>[2x]EERKKELAKEVIETAKKLIEKLAKEE

Several natural systems exhibit ‘facilitated dissociation’, in which an effector (E) can bind to a target–host (TH) complex to form an excited ternary complex (THE)20–26 from which the target dissociates quickly. We set out to design protein systems that undergo facilitated dissociation. We use a switchable target binder (host) and a flexible effector that can rapidly bind to and switch the target–host complex to induce a large steric clash with the target, forming a strained excited ternary complex. We show here that by explicitly considering excited intermediate states when designing coupled protein systems, a broad range of facilitated dissociation systems can be designed.

Because state Y clashes with the target, this conformational change is slow when the target is bound, limiting the rate of effector association and the overall rate of facilitated dissociation. This slow step could be bypassed if the effector could instead first bind to state X and accelerate the transition to state Y. An induced-fit mechanism could provide the driving force: an intrinsically disordered effector could weakly engage with state X, and fold and make more extensive interactions in the strained ternary complex in state Y35, driving the transition in a power-stroke-like motion. The two effectors make nearly identical interactions with AS1, but when unbound, the peptide is disordered whereas the 3hb is structured. In contrast to this induced-fit mechanism of the flexible effector, we find that a rigid effector provides reduced rate acceleration even though it binds more tightly. In kinesin and other biological systems, it is difficult to directly assess the role of flexibility and folding upon binding in overall function; by contrast, our designed model systems allow the direct comparison of flexible and rigid effectors and show that the former yield faster conformational transitions against loads.>[4x]MKVKVGVNGYGTIGKRVAYAVTKQDDMELIGITKTKPDFEAYRAKELGIPVYAASEEFIPRFEKEGFEVAGTLNDLLEKVDIIVDATPGGIGAKNKPLYEKAGVKAIFQGGEKADVAEVSFVAQANYEAALGKNYVRVVSCNTTGLVRTLSAIREYADYVYAVMIRRAADPNDTKRGPINAIKPTVEVPSHHG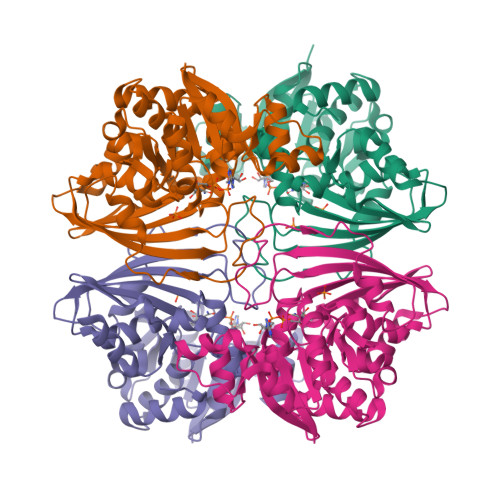PDVQTVIPINIETMAFVVPTTLMHVHSVMVELKKPLTKDDVIDIFENTTRVLLFEKEKGFDSTAQIIEFARDLHREWNNLYEIAVWKESINIKGNRLFYIQAVHQESDVIPENIDAIRAMFELADKWDSIKKTNKSLGILK> MAKATTSVNYACNLDKRLPELPEGANRAQILESTWSTEFKVYDSFGEAHELQIDFARVPGE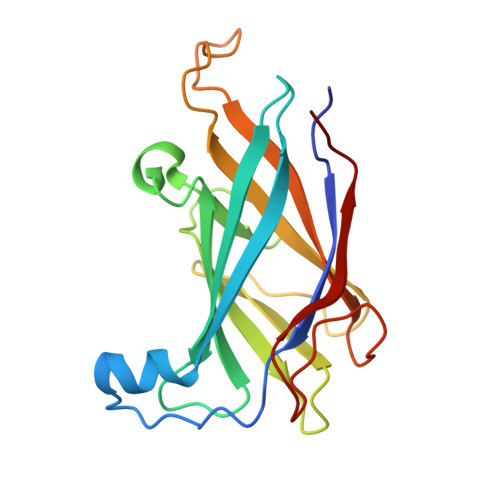VNAWRATVNVDPTNADATATRVGIGTTDGVQNSFIVRFDNNGHLASVTDTAGNVTSPAGQVLVQISYNVVGANPDEAGAPTRHTFDVNLGEIGTSKNTITQFSDKSTTKAYEQDGYT>[4x]GGSNYSADSGNTVYVGNIDPRITKEQLYELFIQINPVLRIKYPKDKVLQAYQGYAFIEFYNQGDAQYAIKIMNNTVRLYDRLIKVRQVTNSTGTTNLPSNIS;>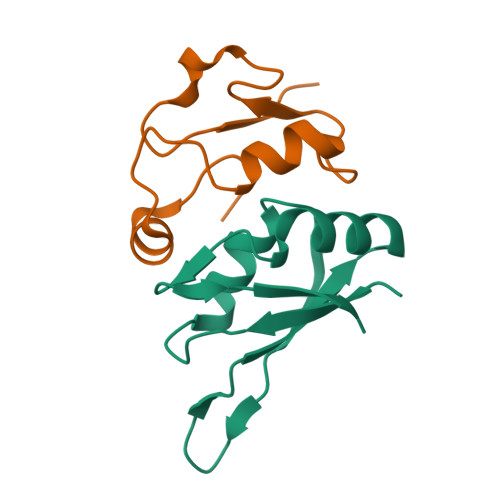MAVGSRPGRISQELRAIMNLPEGQLPPWCMKMKDIGLPTGYPDLKIAGLNWDITNLKGDVYGKIIPNHHSRSKKQGRNYFGALI[4x]(1-HYDROXY-1-PHOSPHONO-2-[1,1';4',1'']TERPHENYL-3-YL-ETHYL)-PHOSPHONIC ACID | C20 H20 O7 P2 | 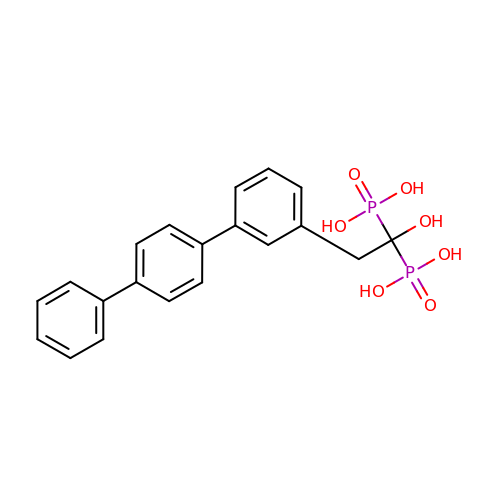MPBUFKZCEBTBSK-UHFFFAOYSA-N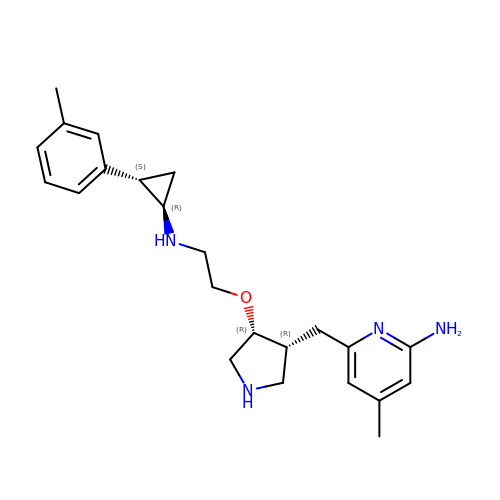4-methyl-6-{[(3R,4R)-4-(2-{[(1R,2S)-2-(3-methylphenyl)cyclopropyl]amino}ethoxy)pyrrolidin-3-yl]methyl}pyridin-2-amine | C23 H32 N4 O | AMEMBWOWTMXVHT-ZDFPQIBNSA-N> MVPGSEGPARAGGLVADVVFVIEGTANLGPYFEELRKHYLLPAIEYFNGGPPAETDFGGDYGGTQYSLVVFNTVDCAPESYVQCHAPTSSAYEFVTWLDGIKFMGGGGESCSLIAEGLSTALQLFDDFKKMREQIGQTHRVCLLICNSPPYLLPAVESTTYSGCTTESLVQKIGERGIHFSIVSPRKLPALRLLFEKAAPPALLEPLQQPADVSQDPRHMVLVRGLVLPVGGSSTSGSLQTKQAVPLPPAPASAATLSAAPPQALPPVPPQYQVPGNLSAAQVAAQNAVEAAKSQKAGLGPRFSPINPLQQAAPGVGPPFSQAPAPPLAPVPPGAPKPPPASQPSLVSTVAPGPVLAAPAQPGAPSLAGTVTPGGVNGPSAAQLGGPALGGQQSVSNKLLAWSGVLEWQEKPKPASVDANTKLTRSLPCQVYVNHGENLKTEQWPQKLIMQLIPQQLLTTLGPLFRNSRMVQFHFTNKDLESLKGLYRIMGNGFAGCVHFPHTAPCEVRVLMLLYSSKKKIFMGLIPYDQSGFVNGIRQVITNH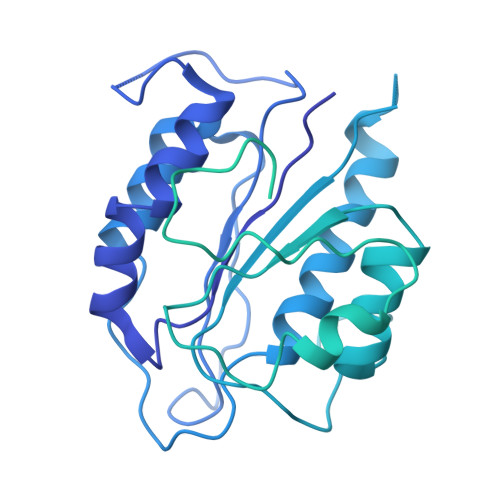KQVQQQKLEQQRGMGAQQAPPVLGPILEEQARPPQNLLQLRAPQPQPQGAVGASAATGQPQPQGATQAPTGAPQGPPGAAPGPPPSGPILRPQNPGANPQLRSLLLNPAPPQTGVPPPQASLHHLQPPGAPTLLPPHQSMGQPQLGPQLLHPPPAQSWPTQLPQRAPLPGQMLLSGGPRGPVPQPGLQPSVMEDDILMDLI> MGSSHHHHHHQNVSLQPPPQQLIVQNKTIDLPAVYQLNGGEEANPHAVKVLKELLSGKQSSKKGMLISIGEKGDKSVRKYSRQIPDHKEGYYLSVNEKEIVLAGNDERGTYYALQTFAQLLKDGKLPEVEIKDYPSVRYRGVVEGFYGTPWSHQARLSQLKFYGKNKMNTYIYGPKDDPYHSAPNWRLPYPDKEAAQLQELVAVANENEVDFVWAIHPGQDIKWNKEDRDLLLAKFEKMYQLGVRSFAVFFDDISGEGTNPQKQAELLNYIDEKFAQVKPDINQLVMCPTEYNKSWSNPNGNYLTTLGDKLNPSIQIMWTGDRVISDITRDGISWINERIKRPAYIWWNFPVSDYVRDHLLLGPVYGNDTTIAKEMSGFVTNPMEHAESSKIAIYSVASYAWNPAKYDTWQTWKDAIRTILPSAAEELECFAMHNSDLGPNGHGYRREESMDIQPAAERFLKAFKEGKNYDKADFETLQYTFERMKESADILLMNTENKPLIVEITPWVHQFKLTAEMGEEVLKMVEGRNESYFLRKYNHVKALQQQMFYIDQTSNQNPYQPGVKTATRVIKPLIDRTFATVVKFFNQKFNAHLDATTDYMPHKMISNVEQIKNLPLQVKANRVLISPANEVVKWAAGNSVEIELDAIYPGENIQINFGKDAPCTWGRLEIS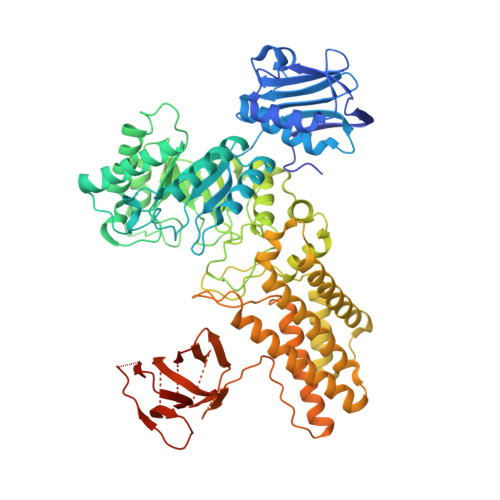TDGKEWKTVDLKQKESRLSAGLQKAPVKFVRFTNVSDEEQQVYLRQFVLTIEKK> AEKQAKINRREEILQALAEMLESNEGASRITTAKLAKQVGVSEAALYRHFPSKTRMFEGLIEFIEESLMSRINRIFDEEKDTL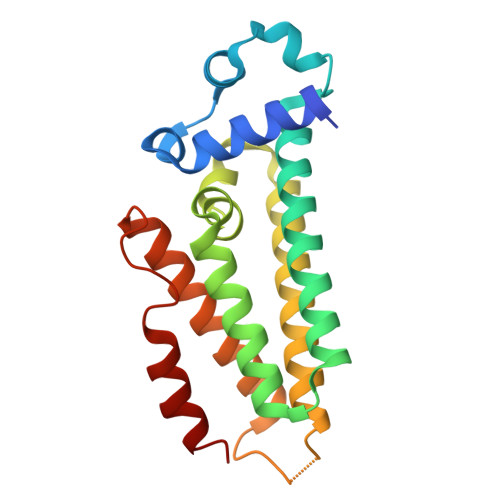NRIRLVMQLLLAFAERNPGLTRILSGHALMFENERLRDRINQLFERIETSLRQILRERKLREGKSFPVDENILAAQLLGQVEGSLNRFVRSDFKYLPTANFDEYWALLSAQIK>GLTPEQKQKKAALSASEGEEVPQDKAPSHVPFLLIGGGTAAFAAARSIRARDPGARVLIVSEDPELPYMRPPLSKELWFSDDPNVTKTLRFKQWNGKERSIYFQPPSFYVSAQDLPHIENGGVAVLTGKKVVQLDVRDNMLKLNDGSQITYEKCLIATGGTPRSLSAIDRAGAEVKSRTTL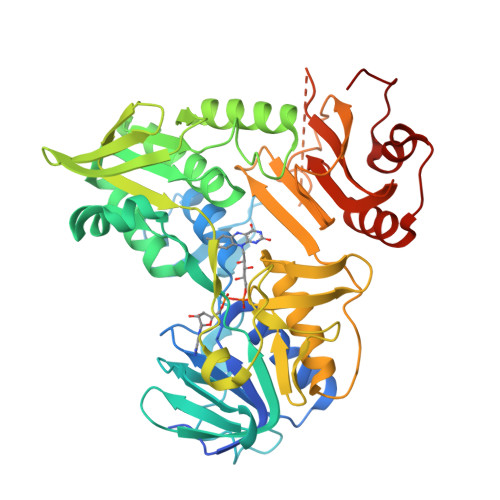FRKIGDFRSLEKISREVKSITIIGGGFLGSELACALGRKARALGTEVIQLFPEKGNMGKILPEYLSNWTMEKVRREGVKVMPNAIVQSVGVSSGKLLIKLKDGRKVETDHIVAAVGLEPNVELAKTGGLEIDSDFGGFRVNAELQARSNIWVAGDAACFYDIKLGRRRVEHHDHAVVSGRLAGENMTGAAKPYWHQSMFWSDLGPDVGYEAIGLVDSSLPTVGVFAKATAQDNPKSATEQSGTGIRSESETESEASEITIPPSTPAVPQAPVQGEDYGKGVIFYLRDKVVVGIVLWNIFNRMPIARKIIKDGEQHEDLNEVAKLFNIHEDLVPR[2x]> DPTECDFELPDLCGWKPDELHDFDWRRLNKKTPSSFLQTGPSYDHTYGKNGSGYYMYIETTGRTENETARLLSPVYDAELAKNGCFIFYYHMYGRGMGGLRVYQKPDRVPMYQLLSSSKRNNYLLFEQWGDQGNEWYSSASMLTDVDDDFQIVIEGIRGNSFMSDIAIDDVSIQRGENCTKAMLHHHHH

The Scavenger Receptor-C (SR-C) and Fibroblast Growth Factor Receptor (FGFR) of Spodoptera frugiperda (Sf-SR-C and Sf-FGFR) have formerly been identified as the cell receptors of Vip3Aa. In 2018, researchers in China found that the scavenger receptor-C (SR-C) of S. frugiperda (Sf-SR-C) is the cell receptor for Vip3Aa. They showed that Sf-SR-C could mediate the toxicity of Vip3Aa through promoting the internalization of Vip3Aa into S. frugiperda cells (Sf9), and that the complement control protein (CCP) domain and MAM domain of Sf-SR-C (Sf-CCP and Sf-MAM) were directly involved in the interaction with Vip3Aa. The Sf-SR-C and Sf-FGFR are single transmembrane proteins in Sf9 cells.

Using X-ray crystallography, we determined the structure of the Sf-MAM domain at a resolution of 2.25 Å. The space group of the structure was P3221. Only one molecule was present in one asymmetric unit. The overall structure contained ten β-strands, which could be divided into three pairs and five short α-helixes. Although the expression construct of the Sf-MAM domain contained three glycosylation sites (Asn186, Asn202 and Asn314), only two glycan chains that linked to the Asn202 and Asn314 residues were built in the final structure. Two disulfide bonds were formed by Cys141-Cys149 and Cys221-Cys315 near both termini of the protein. A calcium atom was present near the N-terminal of the structure. Structure docking analysis of the Sf-MAM and Vip3Aa C-terminal domain (CTD) excluded the possibility of the two proteins binding. The surface plasmon resonance (SPR) assay further demonstrated that the MAM domain of Sf-SR-C and the ectodomain of Sf-FGFR could not bind to the Vip3Aa protein. As some pathogens can invade host cells by binding to scavenger receptors, our structure of the Sf-SR-C MAM domain may provide some insights into insect–pathogen interactions.> TIIETAAAPTEAEIIASGKGKFAWPLRGDIISSFGVKGTGQRNDGLNIRAPQGTPVLSSADGEIAYAGNQVPTFGNLVLVKHADGWVTAYAHLSS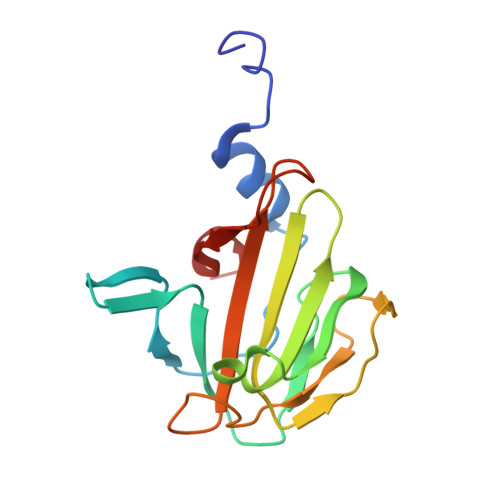TNVKMRQQVKQGEQLGTVGATGGVNEPQLHFEMRYAPTVKDKAKPVDPALVLPR> XYRIPSYDFADKF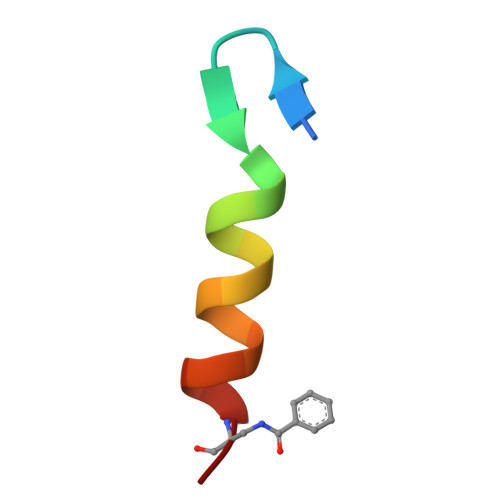KKLLRKAAG>GAMSCIKGNVDLVFLFDGSMSLQPDEFQKILDFMKDVMKKLSNTSYQFAAVQFSTSYKTEFDFSDYVKRKDPDALLKHVKHMLLLTNTFGAINYVATEVFREELGARPDATKVLIIITDGEATDSGNIDAAKDIIRYIIGIGKHFQTKESQETLHKFASKPASEFVKILD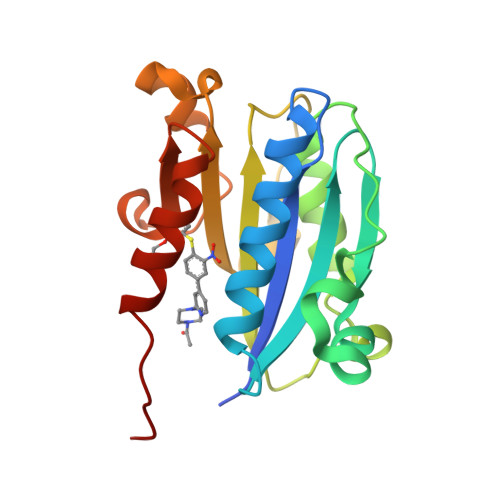TFEKLKDLFTELQKKIYVIEG[4x]>HMLRPVETPTREIKKLDGLWAFSLDRENCGIDQRWWESALQESRAIAVPGSFNDQFADADIRNYAGNVWYQREVFIPKGWAGQRIVLRFDAVTHYGKVWVNNQEVMEHQGGYTPFEADVTPYVIAGKSVRITVCVNNELNWQTIPPGMVITDENGKKKQSYFHDFFNYAGIHRSVMLYTTPNTWVDDITVVTHVAQDCNHASVDWQVVANGDVSVELRDADQQVVATGQGTSGTLQVVNPHLWQPGEGYLYELCVTA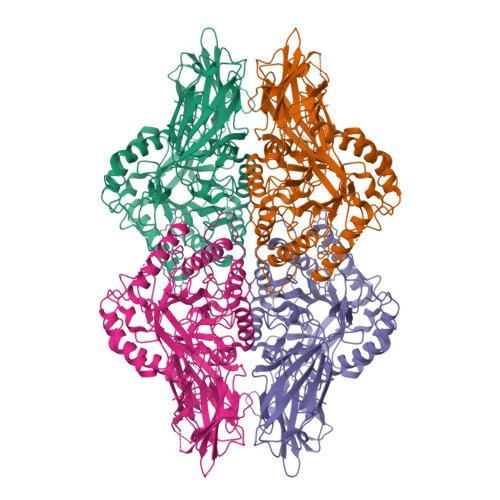KSQTECDIYPLRVGIRSVAVKGEQFLINHKPFYFTGFGRHEDADLRGKGFDNVLMVHDHALMDWIGANSYRTSHYPYAEEMLDWADEHGIVVIDETAAVGFNLSLGIGFEAGNKPKELYSEEAVNGETQQAHLQAIKELIARDKNHPSVVMWSIANEPDTRPQGAREYFAPLAEATRKLDPTRPITCVNVMFCDAHTDTISDLFDVLCLNRYYGWYVQSGDLETAEKVLEKELLAWQEKLHQPIIITEYGVDTLAGLHSMYTDMWSEEYQCAWLDMYHRVFDRVSAVVGEQVWNFADFATSQGILRVGGNKKGIFTRDRKPKSAAFLLQKRWTGMNFGEKPQQGGKQ[2x]Here, we report that a critical glycine residue (Gly463) dominates the motion of threonyl-tRNA synthetase (ThrRS) and the sensitivity of the enzyme to antibiotics. The natural product Obafluorin (OB) is a potent inhibitor of bacterial threonyl-tRNA synthetase (ThrRS). Our previous work showed that OB covalently binds to ThrRS, forming an ester bond with a tyrosine residue in the catalytic center via the highly strained β-lactone ring, making OB the first covalent aaRS inhibitor with demonstrated crystal structures. The binding of OB induces a large conformational change in ThrRS.

To test this speculation, we constructed an EcThrRS_G463A mutant. The TSA experiments showed that OB increased the Tm of EcThrRS_G463A by 19.5 °C, which was 14.0 °C less than that of the WT and 1.3 °C less than the Tm of EcThrRS_G463A increased by 36j. In addition, ATP hydrolysis experiments showed that OB had no inhibitory effect on EcThrRS_G463A, indicating that EcThrRS_G463A is also resistant to OB. In contrast, the conformation of EcThrRS_G463A cannot be further opened, and in this binding mode, OB can be competed out by ATP. Consistent with this assumption, when EcThrRS_G463A was cocrystallized in the presence of both OB and ATP, only ATP was resolved in the pocket. The frequency curve of EcThrRS_G463A had only one peak at a DR-A of approximately 14 Å, which was close to and slightly larger than that of EcThrRS_G463S. This finding suggests that the pocket of EcThrRS_G463A cannot be extended so that its DR-A reaches 17 Å and can be effectively suppressed by OB. Furthermore, by comparing the FEL nadir conformation in the computational simulation and the real crystal structures, we found that the FEL nadir conformation of EcThrRS_WT was closer to the open state crystal structure, while the FEL nadir conformations of EcThrRS_G463S and EcThrRS_G463A were more similar to the apo state crystal structures. These analyses suggest that the G463S and G463A mutations affect the conformational space of the ThrRS structure and cannot expose the active site for OB entry and reaction with Tyr462.

>[2x]MRDHRKIGKQLDLYHMQEEAPGMVFWHNDGWTIFRELEVFVRSKLKEYQYQEVKGPFMMDRVLWEKTGHWDNYKDAMFTTSSENREYCIKPMNCPGHVQIFNQGLKSYRDLPLRMAEFGSCHRNEPSGSLHGLMRVRGFTQDDAHIFCTEEQIRDEVNGCIRLVYDMYSTFGFEKIVVKLSTRPEKRIGSDEMWDRAEADLAVALEENNIPFEYQLGEGAFYAPKIEFTLYDCLDRAWQCGTVQLDFSLPSRLSASYVGEDNERKVPVMIHRAILGSMERFIGILTEEFAGFFPTWLAPVQVVIMNITDSQSEYVNELTQKLSNAGIRVKADLRNEKIGFKIREHTLRRVPYMLVCGDKEVESGKVAVRTRRGKDLGSMDVNEVIEKLQQEIRSRSLKQLEELEHHHHHH> MFLIHFVHYKTILQKYTFKFKHIFLSIDKYNSLFFN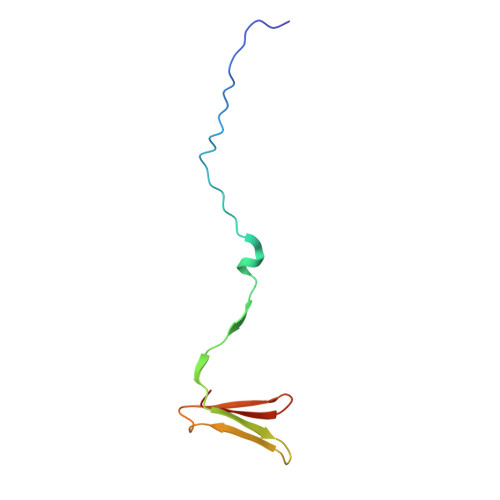ISGILIWLNIIHINIILIKYSFFILINNFEYLIILIST> GCAGCAGC

We have analyzed crystal structures of RNA containing CAG repeats in complex with synthetic cyclic mismatch-binding ligands (CMBLs). In total, three X-ray structures consisting of (GCAGCAGC)2-CMBL3a, one structure of (GCAGCAGC)2-CMBL3b and one (GCAGCAGC)2-CMBL4 complex have been analyzed. The models show well-defined interactions between the molecules in which the CMBLs mimic nucleobases as they form pseudo-canonical base pairs with adenosine residues and engage in extensive stacking interactions with neighboring nucleotides. The binding of ligands is associated with major structural changes of the CAG repeats, which is consistent with results of biochemical studies.

The longer linker contains two N-acyl-amino groups and additional constituents: in CMBL3a it is a E-alkene, in CMBL3b it is an Z-alkene, and in CMBL4 it is an aminoalkyl moiety. One type of interaction includes the typical Watson–Crick pairing and formation of G–C and C–G pairs, which can either fill the voids between duplexes (as in seleno modified CAG(Se)-CMBL3a model) or form short insertions in the pseudo-infinite helical stack (CAG-CMBL4). For CMBL3b and CMBL4, the increases are approximately 6°C and 8°C, respectively. The X-ray structures show that all three ligands interact with the RNA in very similar manners, but the conformation of the bound CMBL3a is the least distorted from the idealized geometry. The asymmetric trans conformation of the long linker makes the ligand better adjusted to the binding site than the symmetric CMBL3b and CMBL4. This is consistent with the thermal melting observations that CMBL3a forms more stable complexes with the RNA than CMBL3b or CMBL4.>[8x]MDHHHHHHLPNITILATGGTIAGGGDSATKSNYTVGKVGVENLVNAVPQLKDIANVKGEQVVNIGSQDMNDNVWLTLAKKINTDCDKTDGFVITHGVDTMEETAYFLDLTVKCDKPVV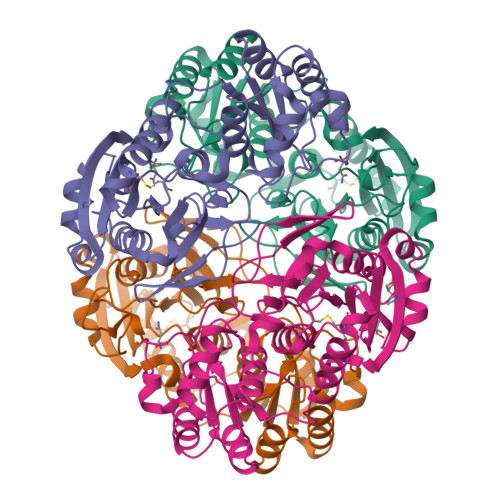MVGAMRPSTSMSADGPFNLYNAVVTAADKASANRGVLVVMNDTVLDGRDVTTTNTTDVATFKSVNYGPLGYIHNGKIDYQRTPARKHTSDTPFDVSKLNELPKVGIVYNYANASDLPAKALVDAGYDGIVSAGVGNGNLYKSVFDTLATAAKTGTAVVRSSRVPTGATTQDAEVDDAKYGFVASGTLNPQKARVLLQLALTQTKDPQQIQQIFNQY5-[3-({[(2,4-DICHLOROBENZOYL)AMINO]CARBONYL}AMINO)-2-METHYLPHENOXY]PENTANOIC 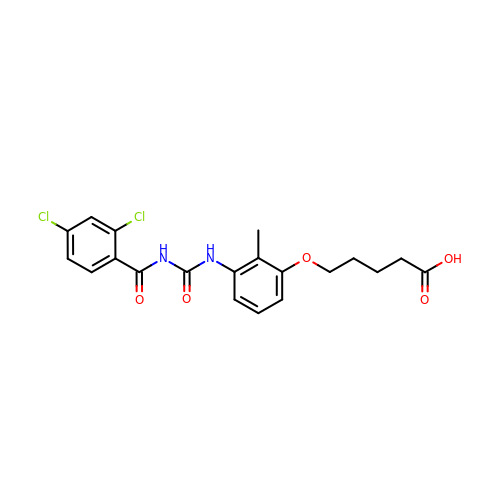ACID | C20 H20 Cl2 N2 O5 | NJJIFGCFUDDBSP-UHFFFAOYSA-N> MTKLKAPAVLAYSRKINPTNALMFAVNWSDRDNTTAVMVGTKTVAGTQSVRGNPNDADKGNIQTVNFANLPHNKNTLLVKYNVKF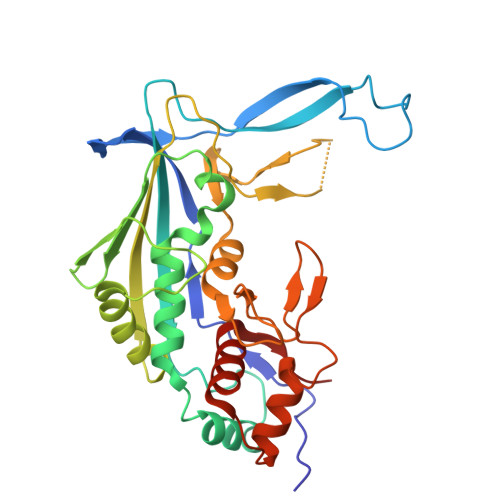VGDVFKAELGGGEYSNTLQTALENTDFGTLAYRYVYNIAAGRTLWRNRVGAESIETVITVNDQTFTFSDLLVNEFDEDVDVAEIADMVAGVLSGEGFVTLKVEHYMLLGEGSEVFPSQEFVENSKLSKQLFDLNGQAAMHDQKIGNAIRTIDTWYEDATTPIAVEPYGSVVRNGVAYRAGNKTDLFTLMDGAVNGKSLTEEDQMFVTANLIRGGVFGGGKD> MLRSSLLPFSYLYEKIINFRNTLYDKGFLKIKKLPVPVISVGNLSVGGSGKTSFVMYLADLLKDKRVCILSRGYKRKSKGTLIVSEYGNLKVSWEEAGDEPYLMAKLLPHVSVVASEDRYKGGLLALEKLSPEVFILDDGFQHRKLHRDLNILLLKKKDLKDRLLPAGNLREPLKEIRRADALVLTYQEVEPFEFFTGKPTFKMFREFCCLLNSDFEEVPFDILKEREVIAFSGLGDNGQFRKVLKNLGIKVKEFMS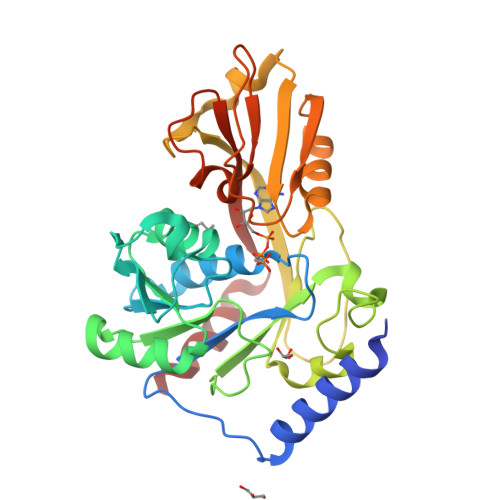FPDHYDYSDFTPEEGEIYLTTPKDLIKLQGYENVFALNFKVKLEREEKLKKLIYRIFY>[3x]TRPNHTIYINNLN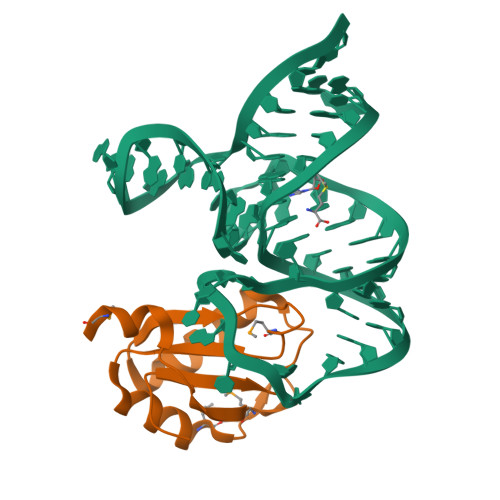EKIKKDELKKSLHAIFSRFGQILDILVKRSLKMRGQAFVIFKEVSSATNALRSMQGFPFYDKPMRIQYAKTDSDIIAKMA> MKKYTCTVCGYIYNPEDGDPDNGVNPGTDFKDIPDDWVCPLCGVGK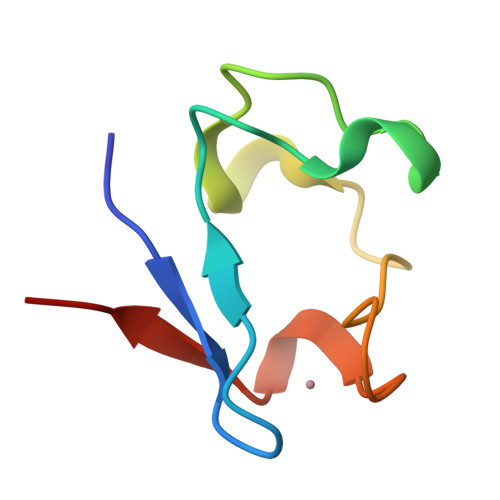DQFEEVEE NsP1 is the membrane anchor for the complex, forming dodecameric pores that associate monotopically with the membrane in the necks of the spherules to gate their entrance. Enzymatically, nsP1 also has a role in addition of cap0 structures to the 5′ end of the positive-sense viral RNAs. NsP1 possesses both N′7 methyltransferase and guanylyltransferase activity and reverses the order of these reactions. Each nsP1 protomer is built around a methyltransferase fold common to SAM-dependent methyltransferases with additional insertions (membrane binding and oligomerisation (MBO) loops 1 and 2) and extensions (ring aperture membrane binding oligomerisation (RAMBO) domain) that contribute to pore formation, oligomerization, and membrane binding.

We finally obtained electron microscopy maps corresponding to the nsP1–m7GMP covalent complex by incubation of the nsP1 protein with the m7GTP and SAH substrates and 27-mer RNA, suggesting that the presence of RNA is able to bypass the metastable state and stimulate the guanylylation reaction. We also obtained a similar structure when substituting the 27-mer by a 15-mer RNA. Here, the position of the guanosine base moves as the ribose and alpha phosphate rotate by 56°, bringing the Pα close enough to H37 for establishing a covalent bond. As a consequence of the phosphate repositioning, residue R41 is now closer to the alpha phosphate and a new H-bond is formed between the ribose and S44 sidechain. In parallel, Y248 is now too far from the alpha phosphate for hydrogen bonding, and sidechains of residues R92 and R275 of the neighboring protomer are no longer visible in the maps. Intriguingly, the SAH substrate remains bound in the SAM binding pocket now extensively contacting by VdW interactions the m7GMP moiety as a consequence of its rotation (from 3 to 14 contacts). There is no density for the pyrophosphate product, suggesting that it leaves with the magnesium ions. The H-bonds of the base with E250, and the ribose with Y285, are maintained despite the rotation of the base. E250, Y285, and R41 appear to be the pivotal residues on which the GMP moiety turns for approaching the catalytic histidine, R41 being next to the Pα transfer reaction site. Transfer of the m7GMP to nsP1 is only observed following incubation with RNA, whether in the form of a capped RNA (in this study and in Zhang et al.) or with uncapped RNA in the presence of m7GTP and SAH (in this study).

>[12x]MDPVYVDIDADSAFLKALQRAYPMFEVEPRQVTPNDXANARAFSHLAIKLIEQEIDPDSTILDIGSAPARRMMSDRKYHCVCPMRSAEDPERLANYARKLASAAGKVLDRNISGKIGDLQAVMAVPDTETPTFCLHTDVSCRQRADVAIYQDVYAVHAPTSLYHQAIKGVRLAYWVGFDTTPFMYNAMAGAYPSYSTNWADEQVLKAKNIGLCSTDLTEGRRGKLSIMRGKKLEPCDRVLFSVGSTLYPESRKLLKSWHLPSVFHLKGKLSFTCRCDTVVSCEGYVVKRITMSPGLYGKTTGYAVTHHADGFLMCKTTDTVDGERVSFSVCTYVPATICDQMTGILATEVTPEDAQKLLVGLNQRIVVNGRTQRNTNTMKNYMIPVVAQAFSKWAKECRKDMEDEKLLGVRERTLTCCCLWAFKKQKTHTVYKRPDTQSIQKVQAEFDSFVVPSLWSSGLSIPLRTRIK>GSHMEPPPKLVLDLERLAHVPQEKAGPLQRYAATIQSQRGAYNGKVLSIRQDDLRTLAVIYDQSPSVLT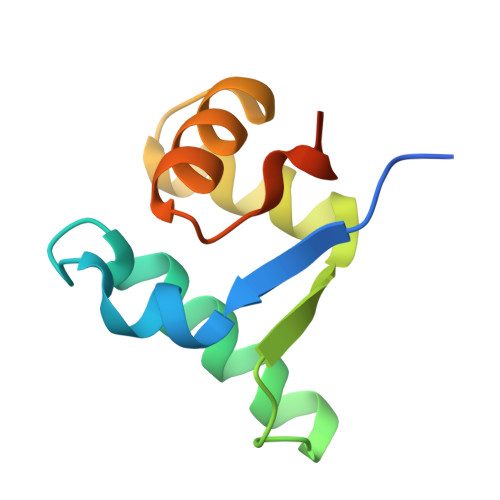EQLISWGVLDADARRAVAHEEN[8x]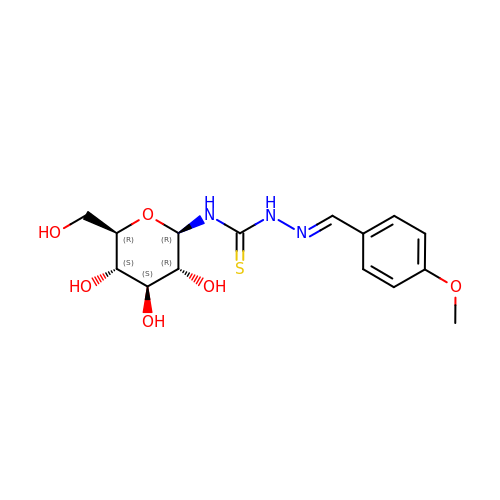N-({(2E)-2-[(4-methoxyphenyl)methylidene]hydrazino}carbonothioyl)-beta-D-glucopyranosylamine | C15 H21 N3 O6 S | GYJJQSIJOBTFIF-VSZQLFBDSA-N>MAAGVPCALVTSCSSVFSGDQLVQHILGTEDLIVEVTSNDAVRFYPWTIDNKYYSADINLCVVPNKFLVTAEIAESVQAFVVYFDSTQKSGLDSVSSWLP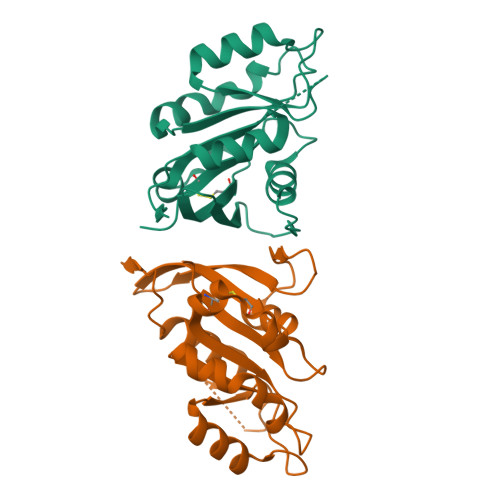LAKAWLPEVMILVCDRVSEDGINRQKAQEWCIKHGFELVELSPKELPEEDDDFPESTGVKRIVQALNANVWSNVVMK[2x]> LPQSVSRAAITAAYRRPETEAVSMLLEQARLPQPVAEQAHKLAYQLADKLRNQKNASGRAGMVQGLLQEFSLSSQEGVALMCLAEALLR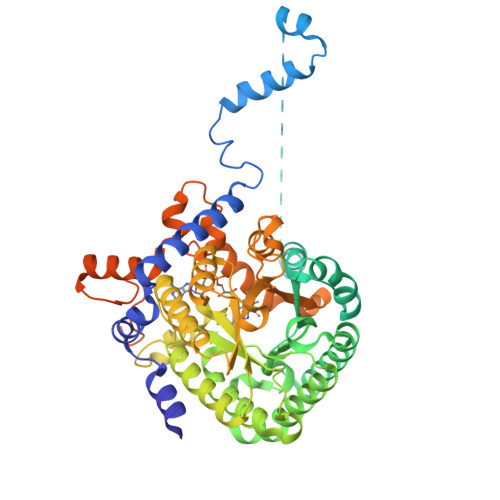IPDKATRDALIRDKISNGNWQSHIGRSPSLFVNAATWGLLFTGKLVSTHNEASLSRSLNRIIGKSGEPLIRKGVDMAMRLMGEQFVTGETIAEALANARKLEEKGFRYSYDMLGEAALTAADAQAYMVSYQQAIHAIGKASNGRGIYEGPGISIKLSALHPRYSRAQYDRVMEELYPRLKSLTLLARQYDIGINIDAEESDRLEISLDLLEKLCFEPELAGWNGIGFVIQAYQKRCPLVIDYLIDLATRSRRRLMIRLVKGAYWDSEIKRAQMDGLEGYPVYTRKVYTDVSYLACAKKLLAVPNLIYPQFATHNAHTLAAIYQLAGQNYYPGQYEFQCLHGMGEPLYEQVTGKVADGKLNRPCRIYAPVGTHETLLAYLVRRLLENGANTSFVNRIADTSLPLDELVADPVTAVEKLAQQEGQTGLPHPKIPLPRDLYGHGRDNSAGLDLANEHRLASLSSALLNSALQKWQALPMLEQPVAAGEMSPVINPAEP> GPLGSNSFVGLRVVAKW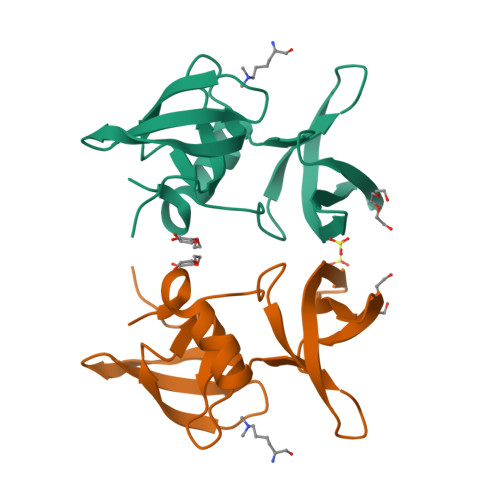SSNGYFYSGKITRDVGAGKYKLLFDDGYECDVLGKDILLCDPIPLDTEVTALSEDEYFSAGVVKGHRKESGELYYSIEKEGQRKWYKRMAVILSLEQGNRLREQYGLG;> SHLKSKKGQST> MAPLYPVLSQASLYKRHFFKNIKLFHVVFYVGAPCVTFGTAAWSGSNRNSREAI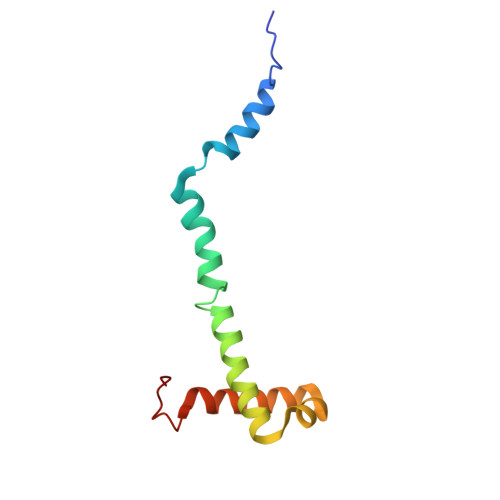FMVIEERHGWDNFKKLSSHQQGVIMQEAAQESLLARNKGELHLP> GAMGSMGVNAVHWFRKGLRLHDNPALRECIQGADTVRCVYILDPWFAGSSNVGINRWRFLLQCLEDLDANLRKLNSRLFVIRGQPADVFPRLFKEWNIAKLSIEYDSEPFGKERDAAIKKLASEAGVEVIVRISHTLYDLDKIIELNGGQPPLTYKRFQTLISRMEPLEMPVETITPEVMKKCTTPVSDDHDEKYGVPSLEELGFDTDGLPSAVWPGGETEALTRLERHLERKAWVANFERPRMNANSLLASPTGLSPYLRFGCLSCRLFYFKLTDLYKKVKKNSSPPLSLYGQLLWREFFYTAATNNPRFDKMEGNPICVQIPWDKNPEALAKWAEGRTGFPWIDAIMTQLRQEGWIHHLARHAVACFLTRGDLWISWEEGMKVFEELLLDADWSVNAGSWMWLSCSSFFQQFFHCYCPVGFGRRTDPNGDYIRRYLPVLRGFPAKYIYDPWNAPESIQKAAKCIIGVNYPKP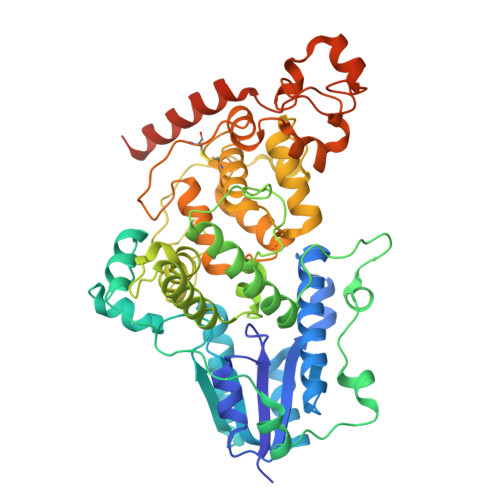MVNHAEASRLNIERMKQIYQQLSRYRGLGLLATVPSNPNGN> AEVLPLTSEWVNRLRNRGYAAYL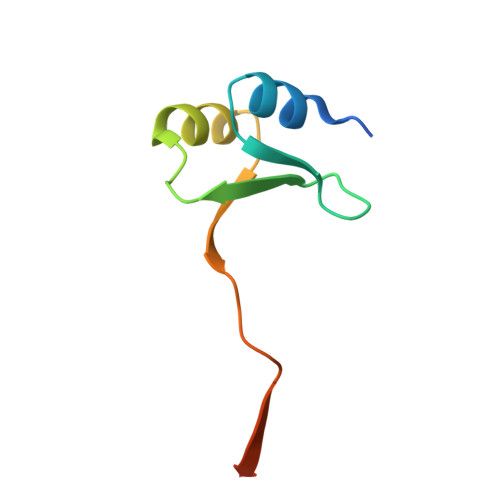SGAGPTAMVLSTEPIPDKVLEDARESGIKVLELEVAGPVKVEVNQPHHHHHH1-(4-cyanophenyl)-3-[[3-(2-cyclopropylethynyl)imidazo[2,1-b][1,3]thiazol-5-yl]methyl]thiourea | C19 H15 N5 S2 | 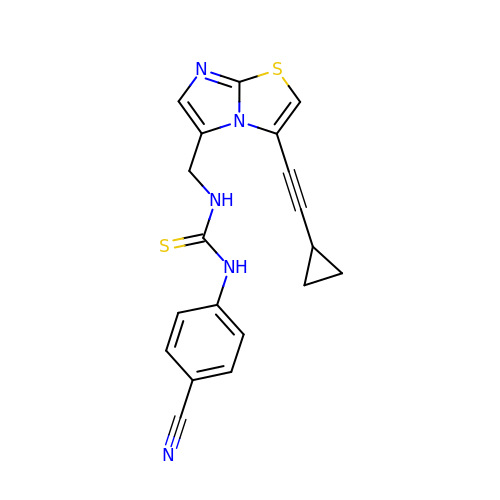OROIVWMQNZZDMT-UHFFFAOYSA-N> MRVLLATCGSRGDTEPLVALAVRVRDLGADVRMCAPPDCAERLAEVGVPHVPVGPSARAPIQRAKPLTAEDVRRFTTEAIATQFDE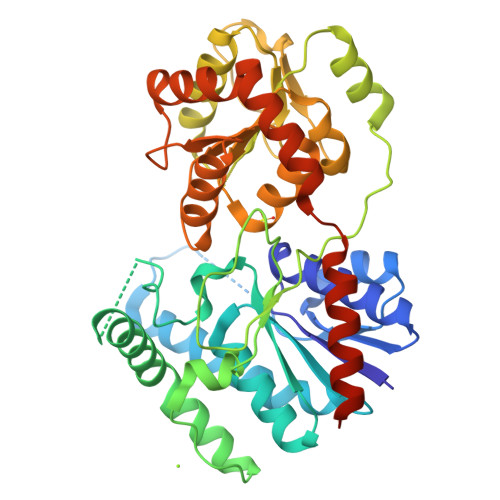IPAAAEGCAAVVTTGLLAAAIGVRSVAEKLGIPYFYAFHCPSYVPSPYYPPPPLGEPSTQDTIDIPAQWERNNQSAYQRYGGLLNSHRDAIGLPPVEDIFTFGYTDHPWVAADPVLAPLQPTDLDAVQTGAWILPDERPLSPELAAFLDAGPPPVYLGFGSLGAPADAVRVAIDAIRAHGRRVILSRGWADLVLPDDGADCFAIGEVNHQVLFGRVAAVIHHGGAGTTHVAARAGAPQILLPQMADQPYYAGRVAELGVGVAHDGPIPTFDSLSAALATALTPETHARATAVAGTIRTDGAAVAARLLLDAVSREKPTVSALEHHHHHH>[4x]MTQFNPVDHPHRRYNPLTGQWILVSPHRAKRPWQGAQETPAKQVLPAHDPDCFLCAGNVRVTGDKNPDYTGTYVFTNDFAALMSDTPDAPESHDPLMR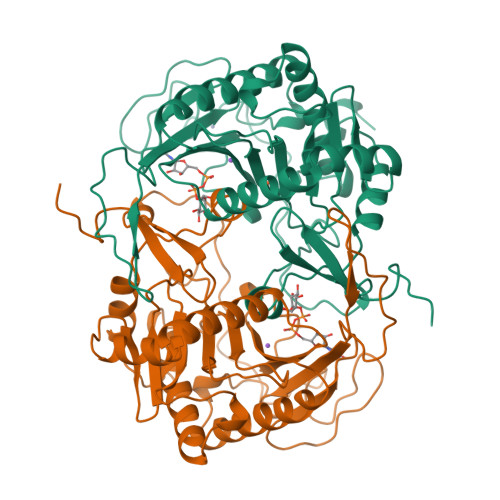CQSARGTSRVICFSPDHSKTLPELSVAALTEIVKTWQEQTAELGKTYPWVQVFENKGAAMGCSNPHPGGQIWANSFLPNEAEREDRLQKEYFAEQKSPMLVDYVQRELADGSRTVVETEHWLAVVPYWAAWPFETLLLPKAHVLRITDLTDAQRSDLALALKKLTSRYDNLFQCSFPYSMGWHGAPFNGEENQHWQLHAHFYPPLLRSATVRKFMVGYEMLAETQRDLTAEQAAERLRAVSDIHFRESGV>[2x]MDYMYGPGRHHLFVPGPVNIPEPVIRAMNRNNEDYRSPAIPALTKTLLEDVKKIFKTTSGTPF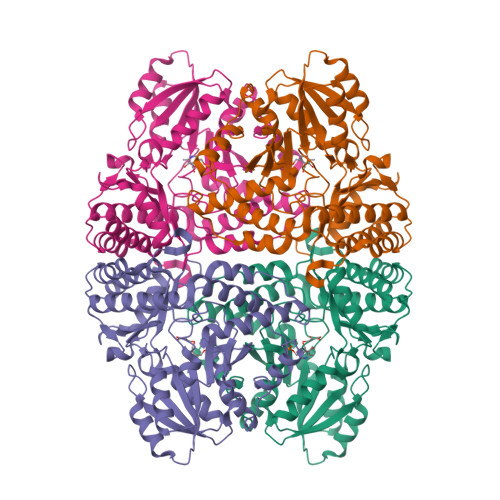LFPTTGTGAWESALTNTLSPGDRIVSFLIGQFSLLWIDQQKRLNFNVDVVESDWGQGANLQVLASKLSQDENHTIKAICIVHNETATGVTNDISAVRTLLDHYKHPALLLVDGVSSICALDFRMDEWGVDVALTGSQKALSLPTGLGIVCASPKALEATKTSKSLKVFFDWNDYLKFYKLGTYWPYTPSIQLLYGLRAALDLIFEEGLENIIARHARLGKATRLAVEAWGLKNCTQKEEWISNTVTAVMVPPHIDGSEIVRRAWQRYNLSLGLGLNKVAGKVFRIGHLGNVNELQLLGCLAGVEMILKDVGYPVVMGSGVAAASTYLQHHIPLIPSRI>SNAQFGGLPVPLDQTLPLNVNPALPLSPTGLAGSLTNALSNALLAEDLLDTLENLPLLDILKPGGGTSGGLLGGLLGKVTSVIPGLNNIIDIKVTDPQLLELGLVQSPDGHRLYVTIPLGIKLQVNTPLVGASLLR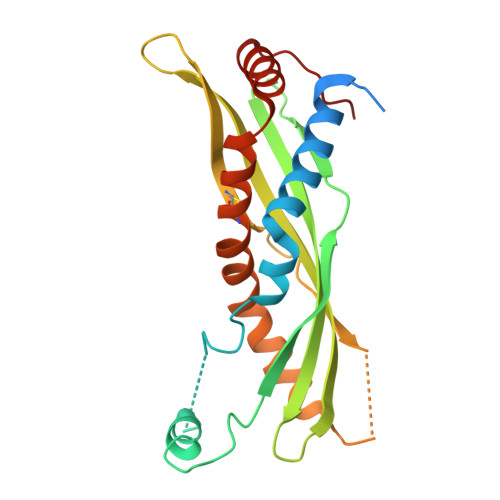LAVKLDITAEILAVRDKQERIHLVLGDCTHSPGSLQISLLDGLGPLPIQGLLDSLTGILNKVLPELVQGNVCPLVNEVLRGLDITLVHDIVNMLIHGLQFVIKV[2x]>[2x]SALAVEADPAADRVSSLSNVSGVLGSQW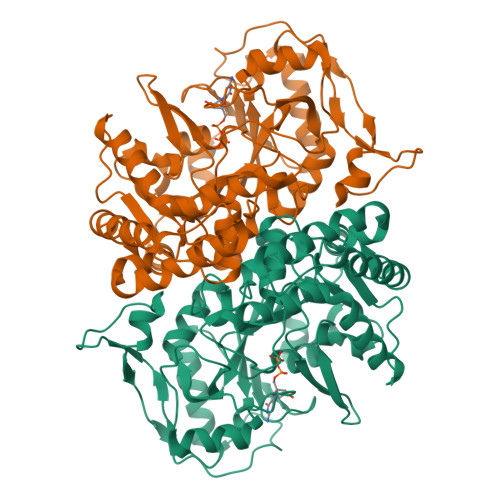GDEGKGKLVDVLAPRFDIVARCQGGANAGHTIYNSEGKKFALHLVPSGILHEGTLCVVGNGAVIHVPGFFGEIDGLQSNGVSCDGRILVSDRAHLLFDLHQTVDGLREAELANSFIGTTKRGIGPCYSSKVTRNGLRVCDLRHMDTFGDKLDVLFEDAAARFEGFKYSKGMLKEEVERYKKFAERLEPFIADTVHVLNESIRQKKKILVEGGQATMLDIDFGTYPFVTSSSPSAGGICTGLGIAPRVIGDLIGVVKAYTTRVGSGPFPTELLGEEGDVLRKAGMEFGTTTGRPRRCGWLDIVALKYCCDINGFSSLNLTKLDVLSGLPEIKLGVSYNQMDGEKLQSFPGDLDTLEQVQVNYEVLPGWDSDISSVRSYSELPQAARRYVERIEELAGVPVHYIGVGPGRDALIYK5,6-dihydroxy-4-oxo-2-phenyl-4H-chromen-7-yl beta-D-glucopyranosiduronic 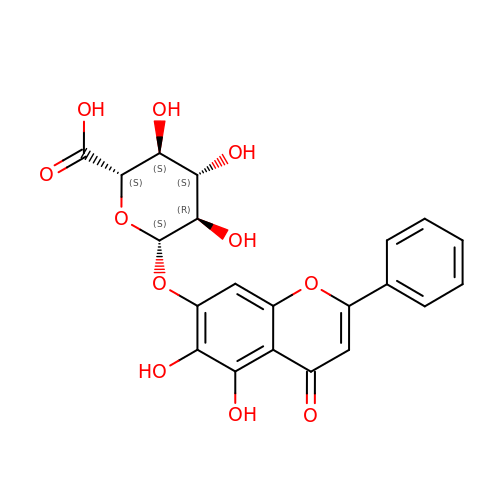acid | C21 H18 O11 | IKIIZLYTISPENI-ZFORQUDYSA-N>KFSVEEYLVHALQGSVSSGQAHSLTSLAKTWAARGSRSREPSPK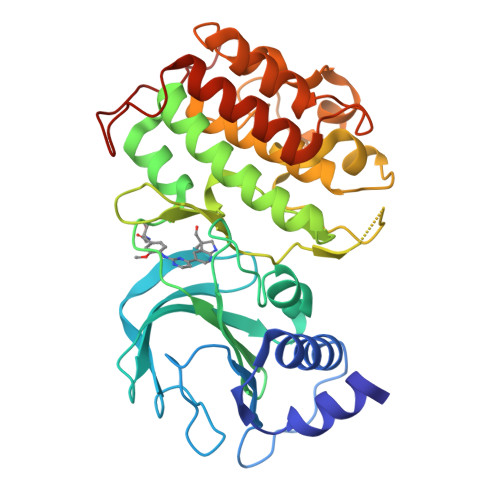TEDNEGVLLTEKLKPVDYEYREEVHWATHQLRLGRGSFGEVHRMEDKQTGFQCAVKKVRLEVFRAEELMACAGLTSPRIVPLYGAVREGPWVNIFMELLEGGSLGQLVKEQGCLPEDRALYYLGQALEGLEYLHSRRILHGDVKADNVLLSSDGSHAALCDFGHAVCLQPDGLGKDLLTGDYIPGTETHMAPEVVLGRSCDAKVDVWSSCCMMLHMLNGCHPWTQFFRGPLCLKIASEPPPVREIPPSCAPLTAQAIQEGLRKEPIHRVSAAELGGKVNRALQQVGGLKSPWRGEYKEPRHPPPNQA[2x]methyl 2-[[[(2~{S})-2-[[3-(trifluoromethyloxy)phenyl]carbamoyl]pyrrolidin-1-yl]carbonylamino]methyl]benzoate | C22 H22 F3 N3 O5 | 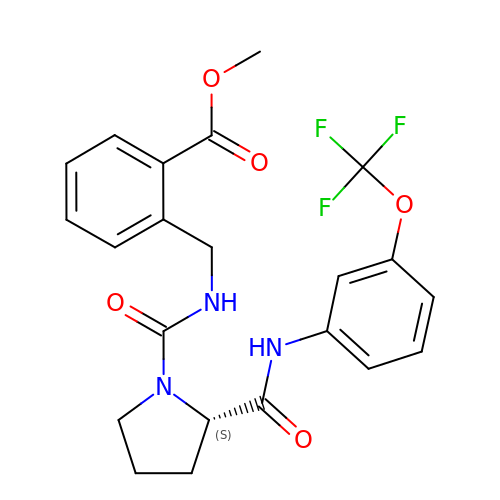PFCVWXAGCYCOIQ-SFHVURJKSA-N> NEAIECHLSDLLQQLTSVNASKPSERGLVRQEEAEDPACIPIFWVSKWVDYSDKYGLGYQLCDNSVGVLFNDSTRLILYNDGDSLQYIERDGTESYLTVSSHPNSLMKKITLLNYFRNYMSEHLLKAGANITPREGDELARLPYLRTWFRTRSAIILHLSNGTVQINFFQDHTKLILCPLMAAVTYINEKRDFQTYRLSLLEEYGCCKELASRLRY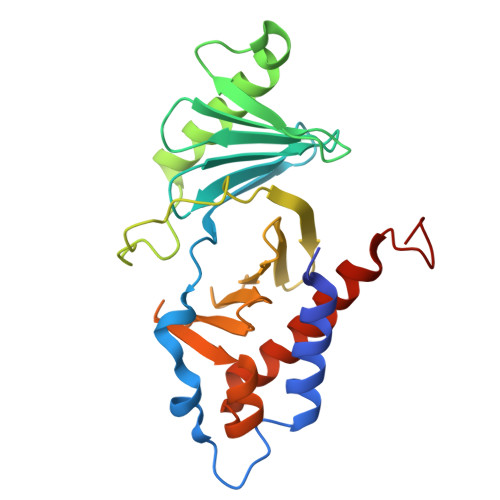ARTMVDKLLSSRSASNRLKAS> GSDTANAPFLCESEQLLIHPKEELSRNNS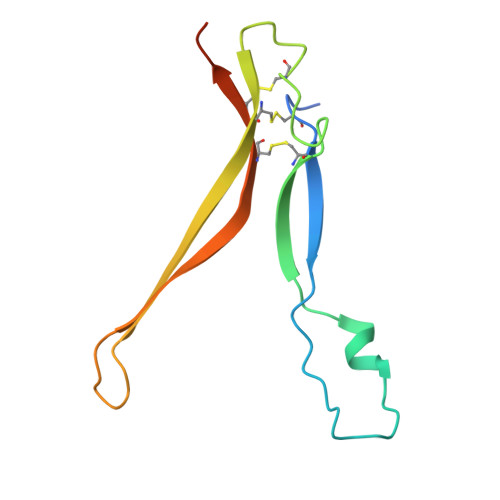MVWIVNTKDYKQGVRIEKCLKRQLGKPCNFCDADTECKQLFHYRTLVAVDKVTKKPYKEQVLLPSCCKCAKILSTGWSHPQFEK S. scabies produces a 200-residue, 22-kDa protein that is a single-domain enzyme called Scabin. Scabin has been cloned, expressed, and purified, and shown to harbor dual enzymatic activities (GH and ADP-ribosyltransferase). Scabin targets DNA as a substrate for ADP-ribose modification; it also shows enzyme specificity towards genomic DNA from Solanum tuberosum tubers. Scabin shares nearly 40% sequence identity with the Pierisin family of mARTs.

Three residues (Trp128, Trp155, and Gln158) bridge the NAD+ and DNA substrates and these were studied and compared to the Scabin WT enzyme. Herein, the fourth-member of this proposed Scabin-NAD+-DNA bridge, Asn110, was investigated with the N110A variant. In Scabin, the Asn to Ala substitution does not perturb enzyme interaction with the NAD+ substrate, since the Michaelis-Menten constant of the N110A variant, KM(εNAD+)N110A = 66 ± 12 μM, is nearly identical to the WT value—KM(εNAD+)WT = 68 ± 3 μM. In Scabin, the Asn to Ala substitution modestly reduces the interaction with ds-DNA, since the dissociation constant of the N110A variant, KD(21bp-DNA)N110A = 82 ± 5 μM, is higher than the KD of the WT toxin of KD(21bp-DNA) = 51 ± 4 μM. The small effect of substitution with Ala on DNA-binding affinity (1.5×) may reflect the small contribution of the Asn110 H-bond to the binding energy. Notably, replacement of Asn110 with Ala severely compromised the enzyme’s ability to transfer ADP-ribose to ss-DNA, making Asn110 an important DNA-transferase residue in Scabin and the fourth member of the Scabin-NAD+-DNA bridge. Given its conservation among the Pierisin family, Asn110 is the new catalytic cornerstone for DNA substrate modification. All the structures were of high quality, ranging from 1.5 to 1.75 Å.

> MGSSHHHHHHSSGENLYFQGSHMTATATSAKAAAPACPRFDDPVHAAADPRVDVERITPDPVWRTTCGTLYRSDSRGPAVVFEQGFLPKDVIDGQYDIESYVLVAQPSPYVSTTYDHDLYKTWYKSGYNYYIDAPGGVDVNKTIGDRHKWADQVEVAFPGGIRTEFVIGVCPVDKKTRTEKMSECVGNPHYEPWH> GDELYRQSLEIISRYLREQATGAKDTKPMGRSGATSRKALETLRRVGDGVQRNHETAFQGMLRKLDIKNEDDVKSLSRVMIHVFSDGVTNWGRIVTLISFGAFVAKHLK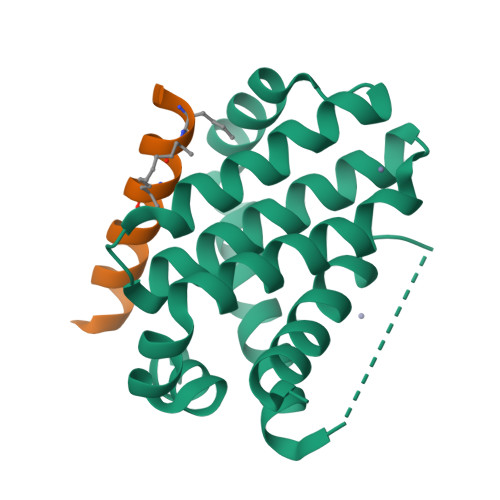TINQESCIEPLAESITDVLVRTKRDWLVKQRGWDGFVEFFHV;> XIWLLQELLRLGDEINARYARX The genomes of most C. perfringens strains contain three separate genes encoding highly conserved GH33 CAZymes targeting sialic acid glycosidic linkages: the nonsecreted 43 kDa NanH, and the two secreted 77 kDa NanI and 129 kDa NanJ. Here, we present the structural and biochemical characterization of the GH33 catalytic domains of the three sialidases of C. perfringens and probe their substrate specificity. The catalytically active domains, which we refer to as NanHGH33, NanJGH33, and NanIGH33, displayed differential activity on various naturally occurring forms of sialic acid. We report the X-ray crystal structures of these domains in complex with relevant sialic acid variants revealing the molecular basis of how each catalytic domain accommodates different sialic acids.

NanJ is highly multimodular comprising a central GH33 domain flanked on the N terminus by family 32 and 40 CBMs and on the C-terminal side by an unknown domain, X82 cohesin, and fibronectin type III-like domains. The positions of the active site residues in the NanJGH33 Neu5,9Ac2 complex remained essentially identical to those in the NanJGH33 Neu5Ac complex, continuing to suggest a relatively rigid active site. The 9-O-Ac group was accommodated by this group being orientated up and away from the active site, rather than continuing the trajectory of the glycerol chain into the a 9-O-Ac binding pocket as in NanHGH33. In NanIGH33 and NanJGH33, the 9-O-Ac binding site is apparently blocked off by phenylalanine residues (F353 and F471 in NanIGH33 and NanJGH33, respectively). The presence of the 9-O-Ac group, however, and how it is positioned in the NanJGH33 active site appears to change the context of other acetyl groups. The conformation of the 9-O-Ac group in the NanJGH33 complex would be anticipated to clash with the conformation of a 7-O-Ac group if positioned in a manner that would allow accommodation in the NanJGH33 active site. NanJGH33 was more efficient than NanIGH33 at hydrolyzing Neu5Gc and could accommodate 7-O-Ac modification, but the latter only when 9-O-acetylation was absent.

> SHMDDVYKTQPVELFYPGYLESRGYRIPALETTKKGTVLASIDVRNNGDHDAPNNNIDVGIRRKEVNGEWEEGKVILDYPGKSAAIDTSLMSATIEENGIEKERIFLIVTHFPEGYGFPNTEGGSGYKEIDGKYYFILKDAQNNEYTVREDGIVYNSEGNETDYVMKNDKTLIQNGEEVGNALLSNSPLKAVGTAHIEMIYSDDDGNTWSEPEDLNPGLKKEWMKFFGTAPGKGIQIKNGEHKGRLVFPIYYTNQNNFQSSAVIYSDDFGETWKLGESPIDTASVSSETVSSGTQLTECQVVEMPNGQLKLFMRNTGSYTRIATSFDGGATWHDEVPEDTSLREPYCQLSVINYSGKINGKDAIIFSNPDASSRVNGSVKVGLINENGTYDNGEPRYEFDWIYNKTVKPGSFAYSCLTELPDGNLGLFYEGEGAGRMAYTEFDLNYLKFNA> VPEAPTPMWPDDLQNHTFLHTVYCQDGSPSVGLSEAYDEDQLFFFDFSQNTRVPRLPEFADWAQEQGDAILFDKEFCEWMIQQIPKLDGKIPVSRGFPIAEVFTLKPLEFGKPNTLVCFVSNLFPPMLTVNWHDHSVPVEGFGPTFVSAVDGLSFQAFSYLNFTPEPSDIFSCIVTHEPDRYTAIAYWVPRNALPSDLLEN;> GGFVAHVESTCLLDDAGTPKDFTYCISFNKDLLTCWDPEENKMAPCNSLANVLSQHLNQKDTLMQ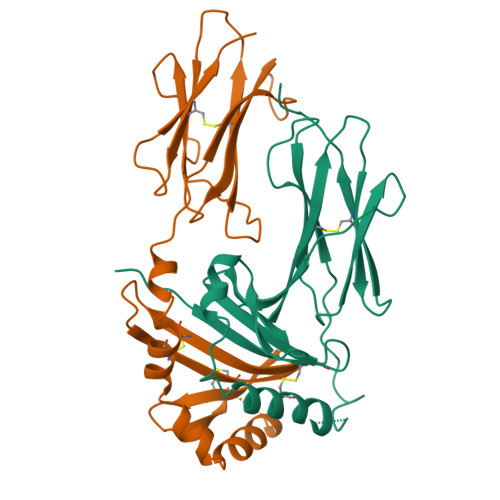RLNGLQNCATHTQPFWGSLTNRTRPPSVQVAKTTPFNTREPVMLACYVWGFYPAEVTITWRKNGKLVMHSSAHKTAQPNGDWTYQTLSHLALTPSYGDTYTCVVEHIGAPEPILRDWTPGLSPMQTLK>[2x]MRVLVRDLKAHVGQEVELLGFLHWRRDLGRIQFLLLRDRSGVVQVVTGGLKLPLPESALRVRGLVVENAKAPGGLEVQAKEVEVLSPALEPTPVEIPKEEWRANPDTLLEYRYVTLRGEKARAPLKVQAALVRGFRRYLDRQDFTEIFTP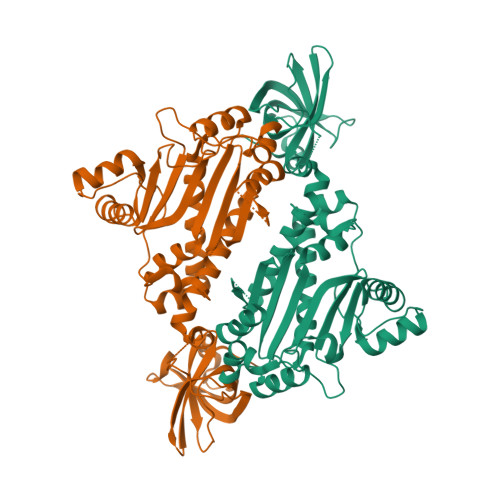KVVRAGAEGGSGLFGVDYFEKRAYLAQSPQLYKQIMVGVFERVYEVAPVWRMEEHHTSRHLNEYLSLDVEMGFIADEEDLMRLEEALLAEMLEEALNTAGDEIRLLGATWPSFPQDIPRLTHAEAKRILKEELGYPVGQDLSEEAERLLGEYAKERWGSDWLFVTRYPRSVRPFYTYPEEDGTTRSFDLLFRGLEITSGGQRIHRYEELLESLKAKGMDPEAFHGYLEVFKYGMPPHGGFAIGAERLTQKLLGLPNVRYARAFPRDRHRLTP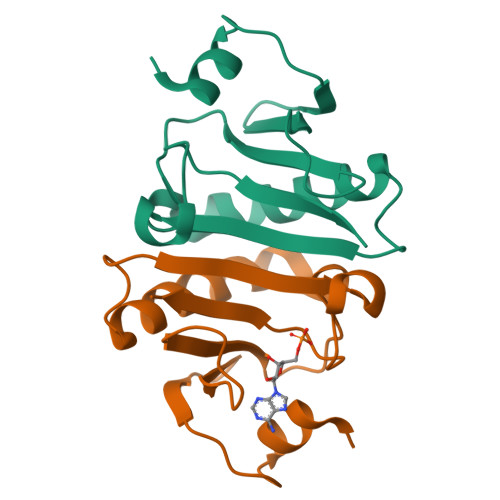>[10x]MNVFEKIIQGEIPCSKILENERFLSFYDINPKAKVHALVIPKQSIQDFNGITPELMAQMTSFIFEVVEKLGIKEKGYKLLTNVGKNAGQEVMHLHFHILSGDKHLEHHHHHH>GPLGSDYIIKEKTVLLQKKDSEGFGFVLRGAKAQTPIEEFTPTPAF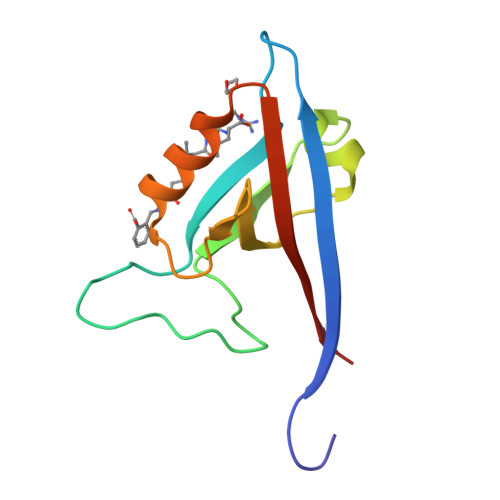PALQYLESVDEGGVAWRAGLRMGDFLIEVNGQNVVKVGHRQVVNMIRQGGNTLMVKVVMVTRHPDM[2x]>SNHHRGLASANVDFAFSLYKHLVALSPKKNIFISPVSISMALAMLSLGTCGHTRAQLLQGLGFNLTE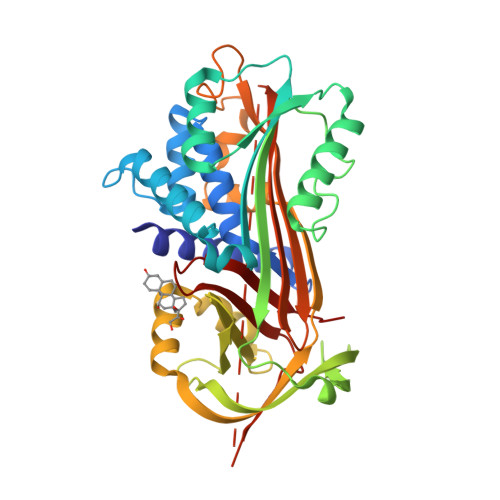RSETEIHQGFQHLHQLFAKSDTSLEMTMGNALFLDGSLELLESFSADIKHYYESEVLAMNFQDWATASRQINSYVKNKTQGKIVDLFSGLDSPAILVLVNYIFFKGTWTQPFDLASTREENFYVDETTVVKVPMMLQSSTISYLHDSELPCQLVQMNYVGNGTVFFILPDKGKMNTVIAALSRDTINRWSAGLTSSQVDLYIPKVTISGVYDLGDVLEEMGIADLFTNQANFSRITQDAQLKSSKVVHKAVLQLNEEGVDTAGSTGVTLNLRSKPIILRFNQPFIIMIFDHFTWSSLFLARVMNPV[4x]The later identification of the kindlin family of proteins revealed them to be key co-activators of integrins, alongside talin. Talin and kindlin interact directly with the cytoplasmic tails of integrin β-subunits, with kindlin binding to a membrane-distal NPxY motif and talin binding to a membrane-proximal NPxY motif. Kindlin-1 is expressed in the epithelial cells of the skin and gut, kindlin-2 is widely expressed but most notably in striated and smooth muscle, and kindlin-3 is expressed particularly in haematopoietic tissues but also in endothelial cells. In any case, membrane binding by kindlins is thus not only an important factor in integrin activation, but may also determine their cell signalling impact and even the cell's fate. The membrane-binding capacity of kindlins has been proved to be essential for integrin activation and is dependent on their PH domains (see Supplementary Figure S1 for a sequence alignment) and on a long loop within the F1 FERM subdomain that is conserved and similar to an equivalent loop in talin.

Here, we report the crystal structure of the kindlin-3 PH domain together with molecular dynamics-based and biophysical characterisation of its inositol phosphate lipid-binding properties. Similar to that of kindlin-1 and -2, the PH domain of kindlin-3 contains an additional C-terminal amphipathic helix extension, which is not present in other PH domains. A salt bridge in the kindlin-1 PH domain (Arg380–Glu416) has been shown to occlude its canonical phosphoinositol-binding site, and in the kindlin-3 PH domain, this salt bridge is replaced by a hydrogen bond (Arg360–Gln396) in the equivalent position. The kindlin-3 PH domain has a mixed surface charge distribution with a pronounced concentration of positive charge at the canonical inositol phosphate-binding site. The kindlin-3 PH domain is closest in structure to the PH domain of kindlin-2 (RMSD = 0.69 Å), with the major conformational difference being in the β1–β2 loop. The PH domains of kindlins-3 and -2 have similar surface charge distribution to the PH domains with canonical inositol phosphate-binding sites, indicating that inositol phosphate might interact in a canonical way through the β1–β2 loop. In particular, the β1–β2 loop is flexible with both simulation force fields, in good agreement with the crystal structure. MD simulation revealed that kindlin-3 PH domain interacts with the PIP lipids primarily via the loop connecting the β1 and β2 strands, and that it has a somewhat higher affinity for binding PtdIns(3,4,5)P3 than for PtdIns(4,5)P2 in a membrane-like system. Moreover, one kindlin-3 PH domain appears to bind multiple inositol phosphate lipids, at both canonical and non-canonical sites, by means of which the affinity of interaction between the PH domain and the membrane is greatly enhanced by an avidity effect.

>[2x]SDLSSGLEVLFQGTDSLTTIPELKDHLRIFRPRKLTLKGYRQYWVVFKDTTLSYYKSQDEAPGDPTQQLNLKGCEVVPDVNVSGQKFCIKLLVPSPEGMSEIYLRCQDEQQYAQWMAACRLASKGRTMADSSYASEVQAILAFLSLQRAG> SINDSKILSLQNKKNALVDTSGYNAEVRVGDNVQLNTIYTNDFKLSSSGDKIIVNLNNNILYSAIYENSSVSFWIKISKDLTNSHNEYTIINSIEQNSGWKLCIRNGNIEWILQDVNRKYKSLIFDYSESLSHTGYTNKWFFVTITNNIMGYMKLYINGELKQSQKIEDLDEVK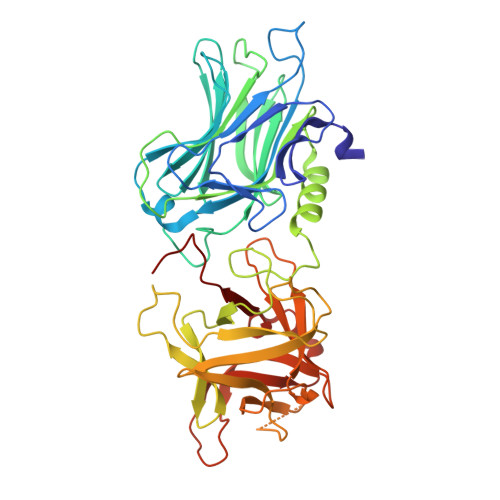LDKTIVFGIDENIDENQMLWIRDFNIFSKELSNEDINIVYEGQILRNVIKDYWGNPLKFDTEYYIINDNYIDRYIAPESNVLVLVQYPDRSKLYTGNPITIKSVSDKNPYSRILNGDNIILHMLYNSRKYMIIRDTDTIYATQGGECSQNCVYALKLQSNLGNYGIGIFSIKNIVSKNKYCSQIFSSFRENTMLLADIYKPWRFSFKNAYTPVAVTNYETKLLSTSSFWKFISRDPGWVE>MSDLKIARIDVFQVDLPYSGGVYYLSAGREYRSFDATIVRITTDTGIEGWGESTPFGSNYIASHPRGVRAGIATMAPSLIGLDPRRVDRINDAMDDALLGHEDAKTAIDVACWDIFGKSVGLPVCELLGGRTNTRLPLISSIYVGEPEDMRARVAKYRAKGYKGQSVKISGEPVTDAKRITAALANQQPDEFFIVDANGKLSVETALRLLRLLPHGLDFALEAPCATWRECISLRRKTDIPIIYDELATNEMSIVKILADDAAEGIDLKISKAGGLTRGR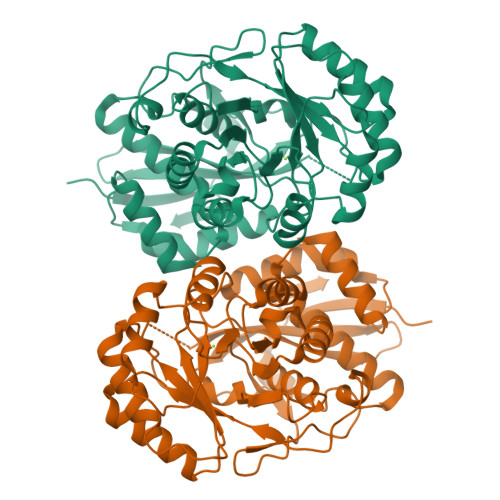RQRDICLAAGYSVSVQETCGSDIAFAAIVHLAQTIPERSLRCILECRDMVTVKTADGAFDIQDGFATAPTTPGLGIMPRLDVLGEAVASYF[4x]>DTGCAIDITRKEMRCGSGIFVHNDVEAWVDRYKYLPETPRSLAKIVHKAHKEGVCGVRSVTRLEHQMWEAVRDELNVLLKENAVDLSVVVNKPVGRYRSAPKRLSMTQEKFEMGWKAWGKSILFAPELANSTFVVDGPETKECPDEHRAWNSMQIEDFGFGITSTRVWLKIREESTDECDGAIIGTAVKGHVAVHSDLSYWIESRYNDTWKLERAVFGEVKSCTWPETHTLWGDGVEESELIIPHTIAGPKSKHNRREGYKTQNQGPWDENGIVLDFDYCPGTKVTITEDCGKRGP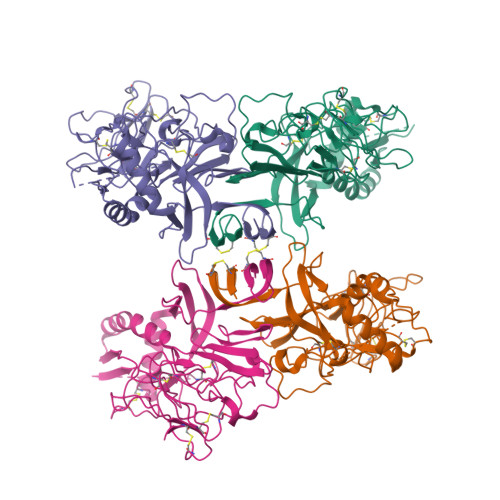SVRTTTDSGKLITDWCCRSCSLPPLRFRTENGCWYGMEIRPVRHDETTLVRSQVDAHHHHHH[4x]>GGRMKFTVEREHLLKPLQQVSGPLGGRPTLPILGNLLLQVADGTLSLTGTDLEMEMVARVALVQPHEPGATTVPARKFFDICRGLPEGAEIAVQLEGERMLVRSGRSRFSLSTLPAADFPNLDDWQSEVEFTLPQATMKRLIEATQFSMAHQDVRYYLNGMLFETEGEELRTVATDGHRLAVCSMPIGQSLPSHSVIVPRKGVIELMRMLDGGDNPLRVQIGSNNIRAHVGDFIFTSKLVDGRFPDYRRVLPKNPDKHLEAGCDLLKQAFARAAILSNEKFRGVRLYVSENQLKITANNPEQEEAEEILDVTYSGAEMEIGFNVSYVLDVLNALKCENVRMMLTDSVSSVQIEDAASQSAAYVVMPMRL[2x]

Griselimycins (GMs) are such promising anti-TB antibiotics that bind and inhibit the mycobacterial DNA polymerase III sliding clamp (DnaN). Although the co-crystal of msDnaN and MP A could not be obtained after intensive attempts, DnaN of E. coli (ecDnaN) was overproduced in E. coli and co-crystallized with MP A, GM and cyclohexyl-GM (CGM). Despite sharing only 29 % sequence identity with msDnaN, the binding pocket of ecDNA shows a sufficient degree of conservation. The binding pocket can be divided into a larger (subsite 1) and a smaller cavity (subsite 2) and as has been shown previously for GM and mycobacterial DnaN, all compounds occupy both subsites of the binding pocket.

The crystal structures were solved at resolutions of 2.12 Å (MP A), 1.65 Å (GM) and 1.50 Å (CGM). MP A was found to bind in the same mode to ecDnaN as GM or CGM. All three substances form hydrogen bonds to only 2 – 3 protein residues, but the additional oxygen in the N-terminal α-keto butyrate residue of MP A provides a second hydrogen bond acceptor for Arg365, which is also conserved in mycobacterial DnaN. The compounds bind mainly via van der Waals interactions with interfaces ranging from 550 Å2 for GM to 590 Å2 for CGM to 600 Å2 for MP A. Compared to available structures of uncomplexed DnaN, only a few residues undergo significant conformational changes upon binding of the compounds - most notably Met362, which has been described to function as a gate between the subsites. The linear, N-terminal part of the ligands in subsite 2 superimposes almost perfectly, while MP A seems to be tilted slightly (approximately 7-10 ° compared to GM/CGM) away from the protein in the region around Pro8. This tilting can be attributed to the longer 5-methyl-l-norleucine residue of MP A at position 6, whereas leucine is present at the same position in GM and CGM. In the complex with msDnaN, GM adopts a conformation very similar to that of MP A in the ecDnaN complex, although GM lacks the 5-methyl-l-norleucine at position 6 and the residues lining the protein pocket around this position are conserved between mycobacteria and E. coli. In comparison to GM and CGM, the higher potency of MP A might be attributed to the increased hydrophobicity of the substance and the larger van der Waals interface with DnaN. The 5-methyl-l-norleucine at position 6 might also play a role by pushing the generally less-tight bound region around Pro8 out of the binding pocket but stabilizing the tighter interaction around the ligand’s bifurcation. The co-crystal structure of ecDnaN bound with MP A and the nanomolar binding affinity of MPs to msDnaN validates DnaN as the molecular target.> MTENNRLSVKLPGLDLKNPIIPASGCFGFGEEYAKYYDLNKLGSIMVKATTLHPRFGNPTPRVAETASGMLNAIGLQNPGLEVIMTEKLPWLNENFPELPIIANVAGSEEADYVAVCAKIGDAANVKAIELNISCPNVKHGGQAFGTDPEVAAALVKACKAVSKVPLYVKLSPNVTDIVPIAKAVEAAGADGLTMINTLMGVRFDLKTRQPILANITGGLSGPAIKPVALKLIHQVAQDVDIPIIGMGGVANAQDVLEMYMAGASAVAVGTANFADPFVCPKIIDKLPELM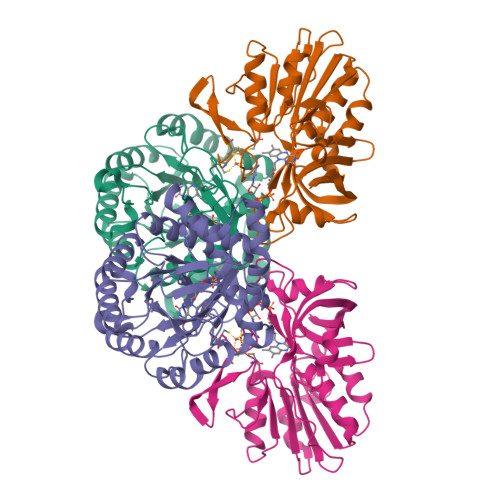DQYRIESLESLIQEVKEGKK;> MSQLQEMMTVVSQREVAYNIFEMVLKGTLVDEMDLPGQFLHLAVPNGAMLLRRPISISSWDKRAKTCTILYRIGDETTGTYKLSKLESGAKVDVMGPLGNGFPVAEVTSTDKILIIGGGIGVPPLYELAKQLEKTGCQMTILLGFASENVKILENEFSNLKNVTLKIATDDGSYGTKGHVGMLMNEIDFEVDALYTCGAPAMLKAVAKKYDQLERLYISMESRMACGIGACYACVEHDKEDESHALKVCEDGPVFLGKQLSL The nsp12 RNA-dependent RNA polymerase possesses some minimal activity on its own6, but the addition of the nsp7 and nsp8 co-factors greatly stimulates polymerase activity. Though additional viral nsp subunits are likely necessary to carry out the full repertoire of replication and transcription activities, the nsp12-nsp7-nsp8 complex so far represents the minimal complex required for nucleotide polymerization. The SARS-CoV RNA-dependent RNA polymerase resembles a cupped right hand with fingers, palm, and thumb subdomains. Although not previously predicted, the SARS-CoV nsp12 contains two metal-binding sites to which we have assigned zinc atoms.

In three-dimensional (3D) classification of the SARS nsp12-nsp7-nsp8 complexes, we observed that a portion of the particles appeared to be missing the nsp7-nsp8 heterodimer. Further 3D sorting and refinement of these particles yielded a reconstruction at 3.5-Å resolution, which largely resembles the larger complex. However, in addition to missing the nsp7-nsp8 heterodimer, this structure also displays a significant amount of disorder in the fingers domain index and ring loops, which play a role in template and NTP binding. We hypothesize that the binding of the nsp7-nsp8 heterodimer to the index finger loop stabilizes the polymerase domain to permit template recognition.

> MGSADASTFLNRVCGVSAARLTPCGTGTSTDVVYRAFDIYNEKVAGFAKFLKTNCCRFQEKDEEGNLLDSYFVVKRHTMSNYQHEETIYNLVKDCPAVAVHDFFKFRVDGDMVPHISRQRLTKYTMADLVYALRHFDEGNCDTLKEILVTYNCCDDDYFNKKDWYDFVENPDILRVYANLGERVRQSLLKTVQFCDAMRDAGIVGVLTLDNQDLNGNWYDFGDFVQVAPGCGVPIVDSYYSLLMPILTLTRALAAESHMDADLAKPLIKWDLLKYDFTEERLCLFDRYFKYWDQTYHPNCINCLDDRCILHCANFNVLFSTVFPPTSFGPLVRKIFVDGVPFVVSTGYHFRELGVVHNQDVNLHSSRLSFKELLVYAADPAMHAASGNLLLDKRTTCFSVAALTNNVAFQTVKPGNFNKDFYDFAVSKGFFKEGSSVELKHFFFAQDGNAAISDYDYYRYNLPTMCDIRQLLFVVEVVDKYFDCYDGGCINANQVIVNNLDKSAGFPFNKWGKARLYYDSMSYEDQDALFAYTKRNVIPTITQMNLKYAISAKNRARTVAGVSICSTMTNRQFHQKLLKSIAATRGATVVIGTSKFYGGWHNMLKTVYSDVETPHLMGWDYPKCDRAMPNMLRIMASLVLARKHNTCCNLSHRFYRLANECAQVLSEMVMCGGSLYVKPGGTSSGDATTAYANSVFNICQAVTANVNALLSTDGNKIADKYVRNLQHRLYECLYRNRDVDHEFVDEFYAYLRKHFSMMILSDDAVVCYNSNYAAQGLVASIKNFKAVLYYQNNVFMSEAKCWTETDLTKGPHEFCSQHTMLVKQGDDYVYLPYPDPSRILGAGCFVDDIVKTDGTLMIERFVSLAIDAYPLTKHPNQEYADVFHLYLQYIRKLHDELTGHMLDMYSVMLTNDNTSRYWEPEFYEAMYTPHTVLLVPRGSGHHHHHHAWSHPQFEK;> AIASEFSSLPSYAAYATAQEAYEQAVANGDSEVVLKKLKKSLNVAKSEFDRDAAMQRKLEKMADQAMTQMYKQARSEDKRAKVTSAMQTMLFTMLRKLDNDALNNIINNARDGCVPLNIIPLTTAAKLMVVVPDYGTYKNTCDGNTFTYASALWEIQQVVDADSKIVQLSEINMDNSPNLAWPLIVTALRANSAVKLQ>[2x]MASSPQRGRPRLNAARTTFVGDNGQPLRGPYTSTEWTAAAPYDQIARVKELGFNAVHLYAECFDPRYPAPGSKAPGYAVNEIDKIVERTRELGLYLVITIGNGANNGNHNAQWARDFWKFYAPRYAKETHVLYEIHNEPVAWGPPYSSSTANPPGAVDMEI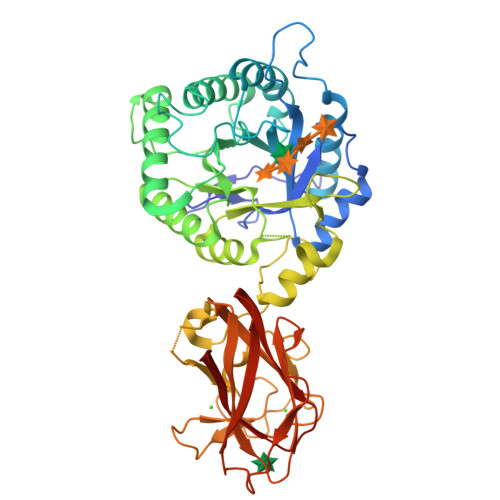DVYRIIRTYAPETPVLLFSYAVFGGKGGAAEALKDIRAFNKAVFGNENAVWTNEAVAFHGYAGWQETTIAVEELLKAGYPCFMTSYAGGAWGSGMGGLDVELTYELERLGVSWLTFQYIPPTGVSDDVTKPEYFSALVENSGLSWTPDYGNWPAARGVYGNGGLARETATWINNFLTGTTRIEAEDFDWGGNGVSYYDTDSVNVGGQYRPDEGVDIEKTSDTGGGYNVGWISEGEWLEYTIRVRNPGYYNLSLRVAGISGSRVQVSFGNQDKTGVWELPATGGFQTWTTATRQVFLGAGLQKLRINALSGGFNLNWIELSPILEHHHHHH> TSDPVRQYLHEIGQVPLLTLEEEIDLARKVEEGMEAIKKLSEATGLDQELIREVVRAKILGTARIQKIPGLKEKPDPKTVEEVDGKLKSLPKELKRYLHIAREGEAARQHLIEANLRLVVSIAKKYTGRGLSFLDLIQEGNQGLIRAVEKFEYKRRFKFSTYATWWIRQAINRAIADQARTIRIPVHMVETINKLSRTARQLQQELGREPSYEEIAEAMGPGWDAKRVEETLKIAQEPVSLETP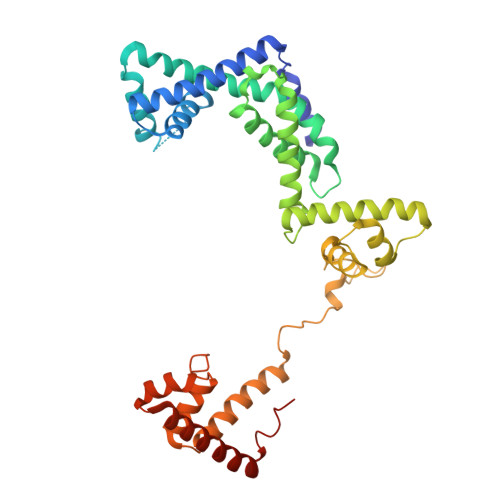IGDEKDSFYGDFIPDENLPSPVEAAAQSLLSEELEKALSKLSEREAMVLKLRKGLIDGREHTLEEVGAYFGVTRERIRQIENKALRKLKYHESRTRKLRDFLE>[2x]SSGAIIYTVELKRYGGPLGITISGTEEPFDPIIISSLTKGGLAERTGAIHIGDRI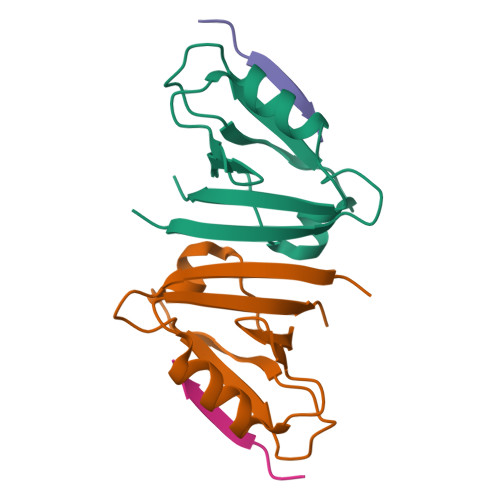LAINSSSLKGKPLSEAIHLLQMAGETVTLKIKKQTDAQPASS;>ATVRTYSC[2x]> MFRRIISNGALLSTQTQRWQDLSKFACLRASLNKESEKAFQELAKKNNVSPQELVELSKIVSMNLDVLKQNINSEQFLLEKESTLKRYRQSSIGTRGHLQTVNEAVNTKYPTLAEGLGQVAGYKEAYQALREIFVHPSISVNNLRQGSYGQQFAVDFRTRADEYVKALLKDHSSNPQAVQTIQEIQHTLHQIIKNYEQNPASIYARILTVLQTRGVNTLPVSKTADQKAVATIQKTSTPSLTIDQLTVPVQERVQTQTVFDAELAFIKEANEMIQQNTGNLPWDGGKKKIFQGQANKYLETPYYLLAALSGLGLLYFLYSGDAKYKTLVLTPVVGIAAFVLLRRNQILNRVPTLTELFLHKDGKFVDAVVSVNGQLISKNDIPVSTLKLYRGDHTVKVNLNDFEDASAKKFLAQQSGQEGVINVHFSKLRNLAA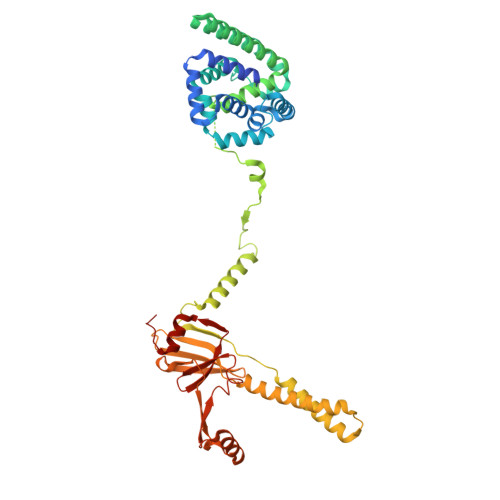RNGQVLNLGDTEVVVPFENQANRIILKQIFKGVEVLPSS Classical Zn2+-dependent deac(et)ylases play fundamental regulatory roles in life and are well characterized in eukaryotes regarding their structures, substrates and physiological roles. Structurally, these enzymes are composed of a central eight-stranded parallel β-sheet flanked by α-helices on each site, known as the α/β-arginase/deacetylase fold. All active site residues were conserved, as shown by the multiple sequence alignment and the structural alignment, suggesting a general acid/base catalytic mechanism for the bacterial enzymes as described for the eukaryotic counterparts. These enzymes mediate catalysis using a penta-coordinated catalytic Zn2+ ion coordinated by two aspartates and a histidine (KpHdaH (1b): Asp181, Asp269, His183).

Overall, the structure of KpHdaH (1b) resembles the structure of P. aeruginosa HdaH solved earlier with an overall r.m.s.d. of 0.41 Å105. All cluster 1 enzymes eluted as apparent trimer or tetramer from the analytical SEC column, and our crystal structures confirmed the formation of tetramers for sub-cluster 1b enzymes. All cluster 1b enzymes contain the so-called L1-loop at the N-terminus as a structural feature mediating the formation of a tetramer via side-by-side arrangement of head-to-head dimers supporting earlier investigations. The L1-loop of each monomer, acting as molecular glue, contacts all three remaining monomers of the tetramers. We postulate restricting the volume of the foot pocket, compared to other bacterial deacylases does not allow longer acyl-chains to be accommodated contributing to restricting the activity to remove acetyl-groups rather than longer acyl-chains. This is mechanistically achieved by the presence of a proline-rich loop, the RPP-motif (general: RPPXHH; KpHdaH: 139-RPPGHH-144; RwDhmhA: 136-RPAGHH-143; RsPrpH: 148-RPAGHH-153). In KpHdaH (1b), RwDhmhA (1b) and RsPrpH (1b), being robust deacetylases, the sequence is EGGY (KpHdaH (1b): 310-EGGY−313) the presence of glutamate further restricting the volume of the foot pocket. Analyses of the surface area surrounding the entry of the active site tunnel shows a highly acidic negatively charged electrostatic surface potential explaining the preference for Arg or Lys at −1 position. As a support, we observed binding of a potassium ion at the negatively charged active site entry in the structure of KpHdaH (1b). Notably, for all sub-cluster 1b enzymes, except for RwDmhA (1b), we found an acetate molecule in the active site coordinating the active site Zn2+ ion.

> MAHHHHHHVGTMKRKTGFFFDERCFWHSTGLHAVTLPVGGWVQPPAGGGHAESPETKRRMKNLMDVSGLTPQLALRSAAPASLEDLRRIHPDSYLERFKAISDNGGGMLGKEAPLGPGSYEIACLSAGLACAAVEAVLKGELDNAYSLSRPPGHHCLPDQSMGFCFLANIPIAVERAKAQLGLGKVAIIDWDVHHGNGTQHIYLQRDDVLTISLHQDGCFPPGYAGEDDRGVGAGEGYNINIPLLAGAGDDSWRYALETIVIPALARFEPELIIIACGYDANAMDPLARMQLHSDSFRAMTEQVQQAADRLCGGKLVMVHEGGYAESYVPFCGLAVMEALSGIRTEVQDPLLEFIQQQQPRATFAQFQRQAIDRLAQQFGLQ L-sorbose | C6 H12 O6 | 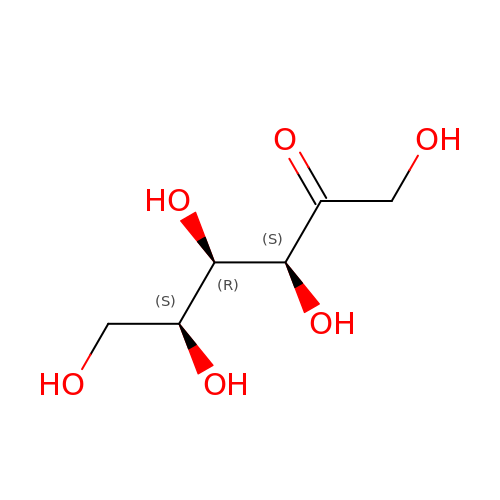BJHIKXHVCXFQLS-OTWZMJIISA-N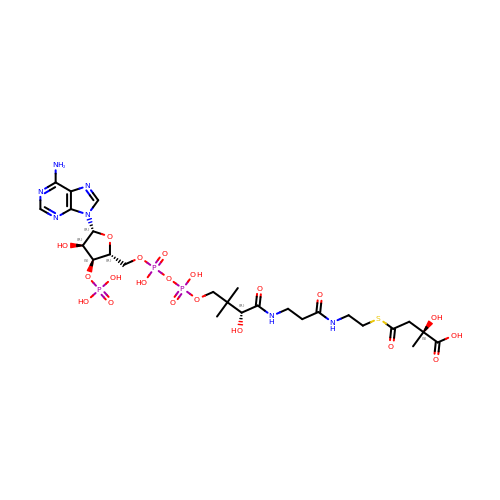Citramalyl-CoA | C26 H42 N7 O20 P3 S | XYGOWHUIVNMEIA-XBVYHAPZSA-N3-[(2~{S},3~{R})-2-carboxypiperidin-3-yl]propyl-$l^{3}-oxidanyl-bis(oxidanyl)boranuide | C9 H19 B N O5 | 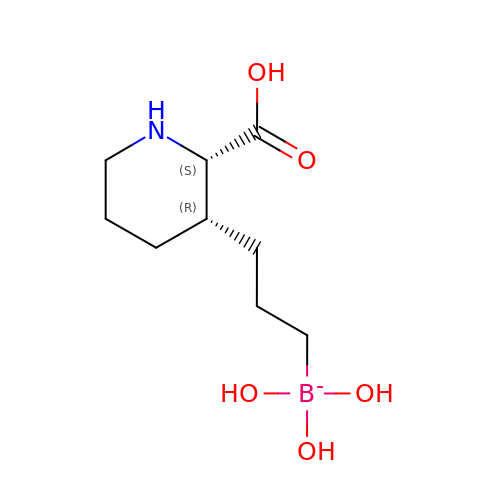WAXQJKOVLQGAHJ-SFYZADRCSA-N>[2x]ASAKLPG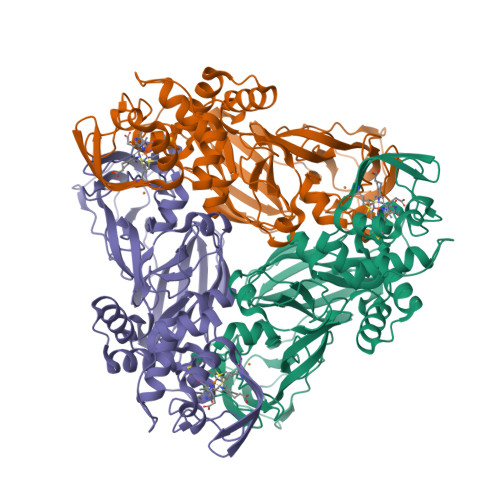DFGPPRGEPIHAVLTSPPLVPPPVNRTYPAKVIVELEVVEKEMQISEGVSYTFWTFGGTVPGSFIRVRQGDTVEFHLKNHPSSKMPHNIDLHGVTGPGGGAASSFTAPGHESQFTFKALNEGIYVYHCATAPVGMHIANGMYGLILVEPPEGLPKVDHEYYVMQGDFYTAGKYREKGLQPFDMEKAIDERPSYVLFNGAEGALTGDKALHAKVGETVRIFVGNGGPNLVSSFHVIGAIFDQVRYEGGTNVQKNVQTTLIPAGGAAVVKFTARVPGSYVLVDHSIFRAFNKGAMAILKIDGAENKLVYSGKELDSVALGDRAAPNMSAVTKATQASVSGTLTVQDQVQAGRALFAGTCSVCHQGNGAGLPGVFPPLAKSDFLAADPKRAMNIVLHGLNGKIKVNGQEYDSVMPPMTQLNDDEVANILTYVLNSWDNPGGRVSAEDVKKVRAQPAPAKAVAEH The subject of this study, the JC virus (JCV), is a member of this family and the causative agent of a brain disease termed Progressive Multifocal Leukoencephalopathy (PML), a disease that is often fatal and for which there is no cure. Herein we present the high-resolution crystal structure of the origin binding domain (OBD) from the JCV initiator protein large T-antigen. The T-antigens encoded by polyomaviruses are multi-domain, multifunctional proteins that form hexamers and double hexamers at origins of replication. The topology of the JCV OBD is a five-stranded antiparallel β-sheet sandwiched between two helices on either side.

The JCV OBD (residues 132–261) crystallized in three different forms that were termed form 1, form 2 and form 3. The four structures are very similar; a superposition of the four JCV OBD structures revealed root mean-squared deviations (RMSDs) of less than 0.5 Å. JCV OBD region B3 (residues 216–220) is poorly ordered in crystal forms 1 and 2, but well ordered in form 3. This loop is also poorly ordered in several of the SV40 OBD structures. To better understand how the JCV T-ag OBDs may assemble during oligomerization, we examined the interactions among the OBDs within the three crystal forms. As described in this section, the largest interface between adjacent molecules is the same in all three crystals. To extend these analyses, we examined the interactions among OBDs within crystal forms 2 and 3. Therefore, crystal forms 2 and 3 were superimposed on one OBD from crystal form 1 and the relevant symmetry mates displayed (crystal form 1 is colored as in Fig. 8A, while the other two forms are colored gray). Furthermore, the near perfect superposition indicates that the interfaces are nearly identical. In addition, crystal forms 2 and 3 also formed a right-handed tetrameric spiral (data not shown).

> GSKVEDPKDFPVDLHAFLSQAVFSNRTVASFAVYTTKEKAQILYKKLMEKYSVTFISRHGFGGHNILFFLTPHRHRVSAINNYCQKLCTFSFLICKGVNKEYLFYSALCRQPYAVVEESIQGGLKEHDFNPE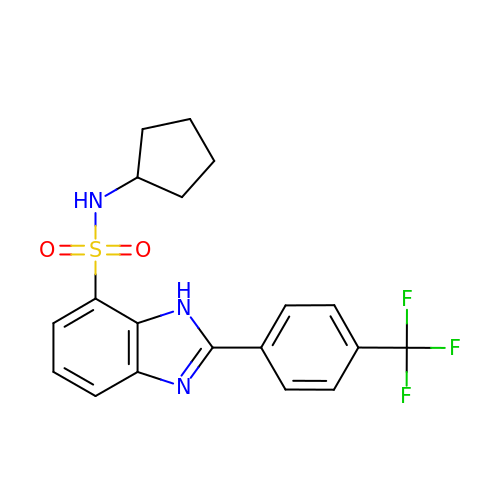N-cyclopentyl-2-[4-(trifluoromethyl)phenyl]-3H-benzimidazole-4-sulfonamide | C19 H18 F3 N3 O2 S | BCAADIRANQOVRJ-UHFFFAOYSA-N>[4x]GSTGSAEELRTLLNKSNVYALAAGSLNPYYKRTIMMNEYRAKAALKKN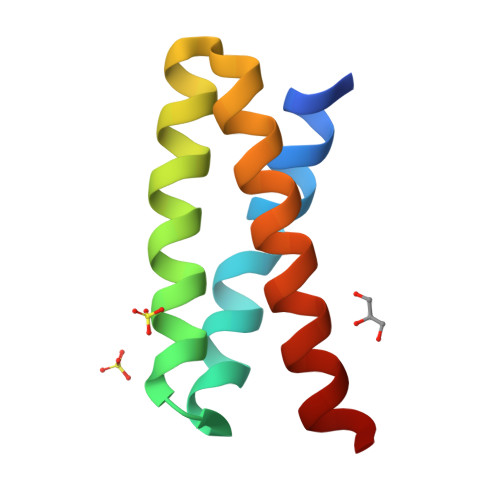DFVSMADAKVALEKIYKEIDEIINR Endolysins are bacteriophage lytic enzymes that can hydrolyze cell wall peptidoglycan, causing lysis and bacterial cell death. The LysECD7 is predicted to be a zinc-binding metallopeptidase with L-alanyl-D-glutamate endopeptidase activity (cd14845) cleaving the peptidoglycan (PG) stem peptide. LysECD7 reveals a wide spectrum of activity against Gram-negative bacterial species, but it is not stable enough in PBS and human blood sera. Thus, this molecule was modified with the N-terminal α-helix of SMAP cationic peptide to enhance the antimicrobial properties, suggesting SMAP-mediated permeabilizing activity of the fusion.

The active center of the enzyme contains three amino acids coordinating Zn2+ ion (H62, D69 and H117) and two additional charged acids (R41 and D114) bound to the water molecule for Zn2+ coordination, forming a charged groove important for PG binding. LysECD7 also contains the SxHxxGxAxD motif (60–69 aa) in the cleft region conserved for LAS-type enzymes. For endolysins acting against Gram-negative bacteria, the presence of an additional membrane-translocating domain is predicted, allowing the enzymes to cross the outer membrane of bacteria and reach the peptidoglycan substrate. There is no obvious characteristic sequence on the ether C- or N-terminus of LysECD7, but a region enriched in charged and polar amino acids is detected in the α2 helix around 44–61 aa of the chain, predicted to be intrinsically-disorder region (IDR) with strong polyampholytic properties (FCR = 0.44) and low overall hydrophobicity (2.76), also containing a putative antimicrobial peptide. It forms a protrusion covering the substrate binding pocket of the enzyme and is enriched in lysine residues along the inner surface. Such elements can lack a compact ordered structure, e.g., under conditions of neutral pH in vitro, while under certain conditions the structure is stabilized and the domain acquires functionality, either the IDR can fold upon binding to interaction partners such as PG and other bacterial cell membrane structures. Comparison of the solved structures of native and hybrid molecules revealed only a slight difference in two α-helices involving α2 and α5, which together with the β1-β3 sheet form peptidoglycan-binding pocket, resulting in a more closed cleft architecture of LysECD7-SMAP. We could not resolve the SMAP peptide structure, due to its high mobility, thus the LysECD7-SMAP model was used to perform molecular dynamics simulations. During the simulation the ‘core’ LysECD7 part remains stable (residues 1–131), while the structure of SMAP fragment is remarkably variable (residues 132–148), proposing the free interaction with bacterial membranes. Considering that unmodified LysECD7 lacks activity against other Gram-positive bacteria, e.g. S. aureus, we propose the substrate specificity towards A1γ-type peptidoglycan stem peptides specific for Bacillus spp. and most Gram-negative species.

> MFKLSQRSKDRLVGVHPDLVKVVHRALELTPVDFGITEGVRSLETQKKYVAEGKSKTMKSRHLHGLAVDVVAYPKDKDTWNMKYYRMIADAFKQAGRELGVSVEWGGDWVSFKDGVHFQLPHSKYPDPKLEHHHHHHHH> GGGRGRLILEHTLQGHKGRIWGVAWHPKGNVFASCGEDKAIRIWSLTGNTWSTKTILSDGHKRTIREIRWSPCGQYLASASFDATTAIWSKSSGEFECNATLEGHENEVKSVSWSRSGGLLATCSRDKSVWIWEVAGDDEFECAAVLNPHTQDVKRVVWHPTKDILASASYDNTIKMFAEEPIDNDWDCTATLTSHTSTVWGIDFDADGERLVSCSDDTTIKIWRAYH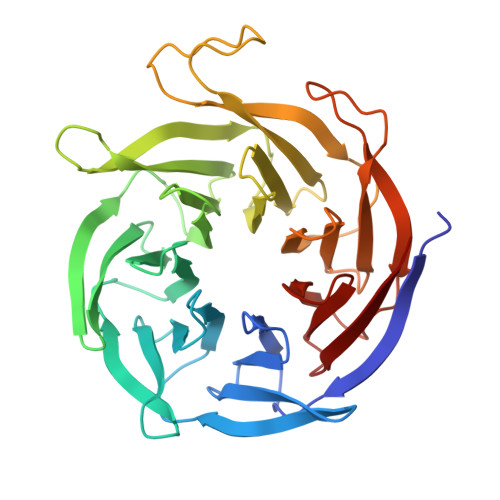PGNTAGVATPDQQTVWKCVCTVSGQHSRAIYDVSWCKLTGLIATACGDDGIRIFKESSDSKPDEPTFEQITAEEGAHDQDVNSVQWNPVVAGQLISCSDDGTIKIWKVTE>SDEINAQSVWSEEISSNYPLCIKNLMEGLKKNHHLRYYGRQQLSLFLKGIGLSADEALKFWSEAFTNMTMEKFNKEYRYSFRHNYGLEGNRINYKPWDCHTILSKPRPGRGDYHGCPFRDWSHERLSAELRSMKLTQAQIISVLDSCQKGEYTIACTKVFEMTHNSASADLEIGEQTHIAH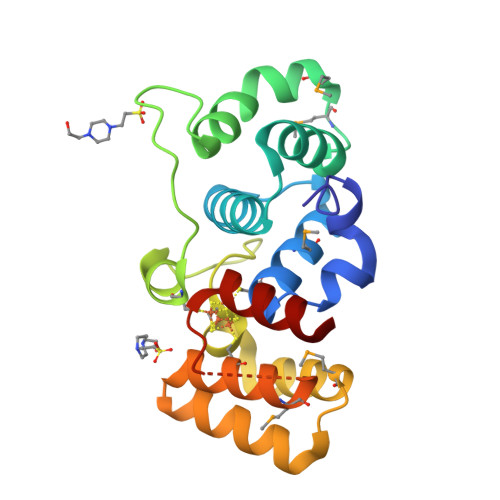PNLYFERSRQLQK[2x]5-oxidanyl-1H-pyridin-2-one | C5 H5 N O2 | 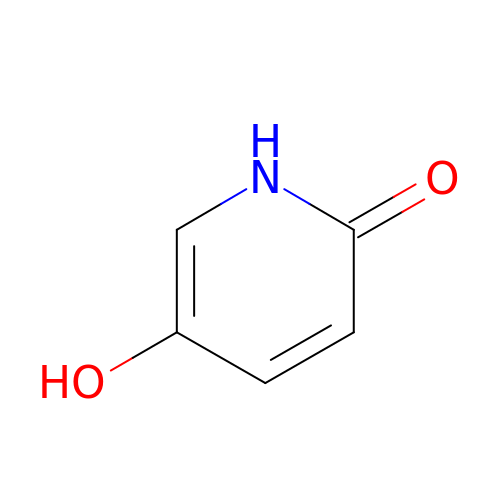CHGPEDOMXOLANF-UHFFFAOYSA-N>[2x]GDTKEQRIL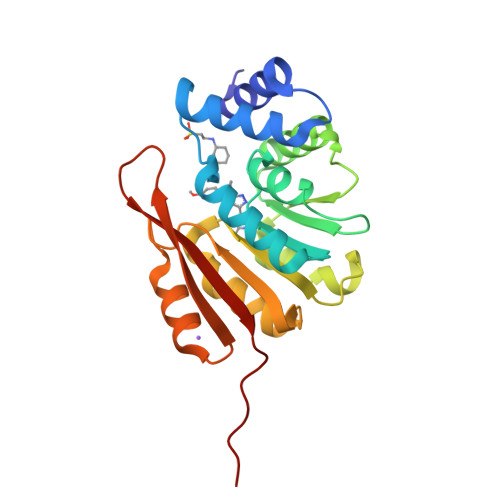RYVQQNAKPGDPQSVLEAIDTYCTQKEWAMNVGDAKGQIMDAVIREYSPSLVLELGAYCGYSAVRMARLLQPGARLLTMEINPDCAAITQQMLNFAGLQDKVTILNGASQDLIPQLKKKYDVDTLDMVFLDHWKDRYLPDTLLLEECGLLRKGTVLLADNVIVPGTPDFLAYVRGSSSFECTHYSSYLEYMKVVDGLEKAIYQGPSSPDKS2-[(2-phenoxyethyl)sulfanyl]-1H-benzimidazole | C15 H14 N2 O S | 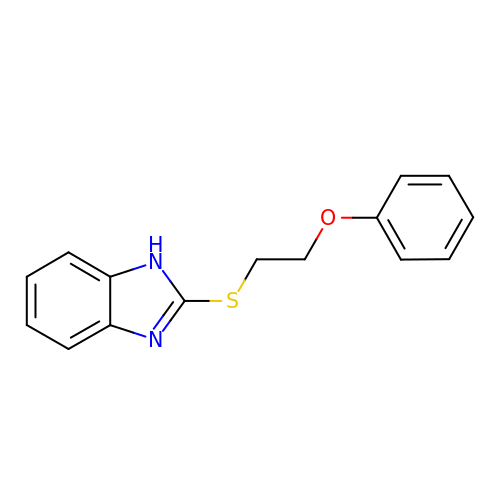UEYUFQWEHMSHIX-UHFFFAOYSA-N>[2x]GHMNVAKREFIRGMMAHYRASLPPPEHSVVIHELQKRVLDIGMLAVNKAHVELFGSHVSGFCTPHSDADISLTYRNFSPWLQGMERVDEQNNKRMTRFGKEASAMGMEDVRYIRARIPVVQFTDGVTGIHCDVSIGNIGGVENSKILCAIRQVFPDFYGAYIHLVK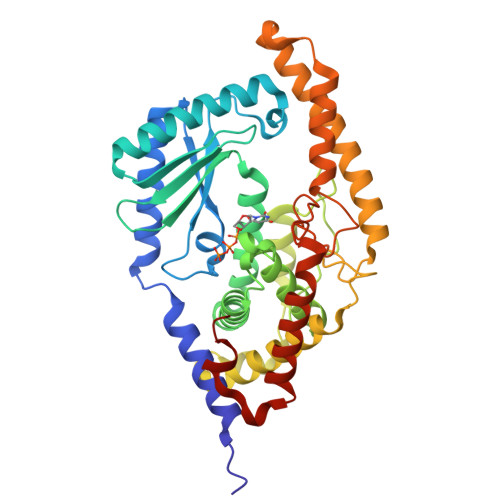AWGKAREVIAPERSTFNSFTVTTMALMVLQELGLLPVFSKPTGEFGELTVADAEMLLQEFKLPPIYDSLHDDDEKLGEAVFFCLQRFAEYYAKYDFSAGTVSLIHPRRHRTVYERVVRRHLELLGSRKRLEWEKHIAEHKEDGPLDENDFSASMQNETTQRPSNSPYVVEDFVNYVNCGRRVQASRVRHIQQEFNRLREMLIDKESELKFDEVFRESDTVP OCTANEDIOIC ACID HYDROXYAMIDE 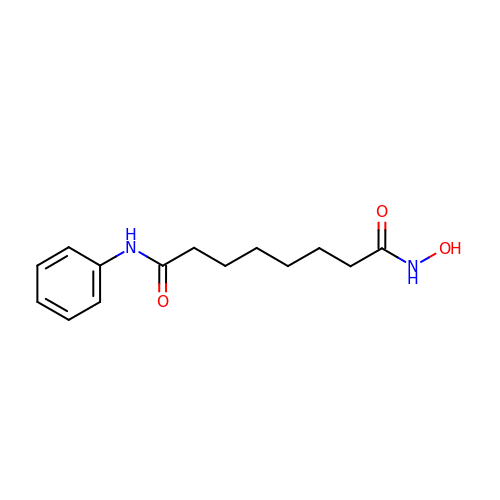PHENYLAMIDE | C14 H20 N2 O3 | WAEXFXRVDQXREF-UHFFFAOYSA-N>MLIMHQVVCAT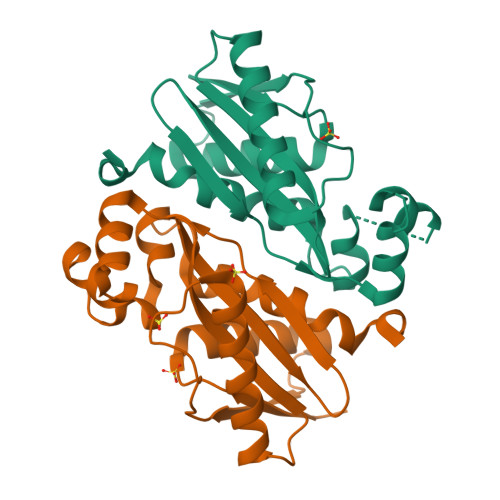TNPAKIQAILQAFHEIFGEGSCHIASVAVESGVPEQPFGSEETRAGARNRVANARRLLPEADFWVAIEAGIDGDSTFSWVVIENASQRGEARSATLPLPAVILEKVREGEALGPVMSRYTGIDEIGRKEGAIGVFTAGKLTRASVYHQAVILALSPFHNAVYSGRVEHHHHHH[8x]> MALRGTVTDFSGFDGRADAEVLRKAMKGLGTDEDSILNLLTARSNAQRQQIAEEFKTLFGRDLVNDMKSELTGKFEKLIVALMKPSRLYDAYELKHALKGAGTDEKVLTEIIASRTPEELRAIKQAYEEEYGSNLEDDVVGDTSGYYQEMLVVLLQANRDPDTAIDDAQVELDAQALFQAGELKWGTDEEKFITILGTRSVSHLRRVFDKYMTISGFQIEETIDRETSGNLENLLLAVVKSIRSIPAYLAETLYYAMKGAGTDDHTLI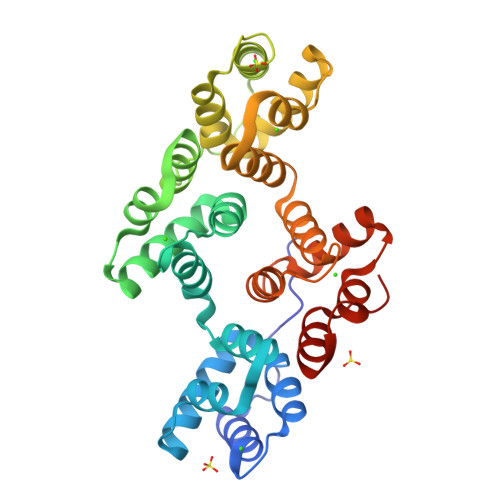RVIVSRSEIDLFNIRKEFRKNFATSLYSMIKGDTSGDYKKALLLLCGGEDD(2S,3R)-2-benzyl-3-sulfanylbutanoic acid | C11 H14 O2 S | 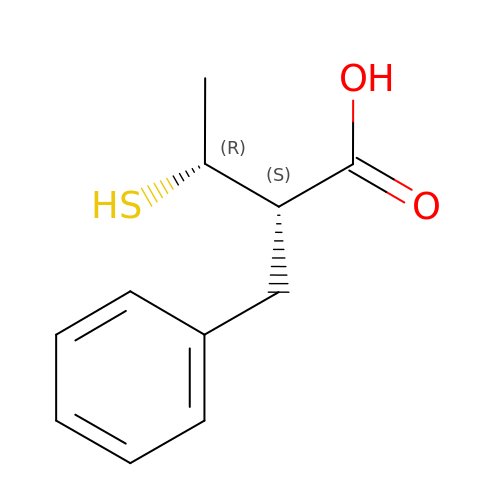LYLMADGMEFUMHJ-PSASIEDQSA-N>FLGDGGDVSFSTRGTQNWTVERLLQAHRQLEERGYVFVGYHGTFLEAAQSIVFGGVRARSQDLDAIWRGFYIAGDPALAYGYAQDQEPDARGRIRNGALLRVYVPRSSLPGFYRTSLTLAAPEAAGEVERLIG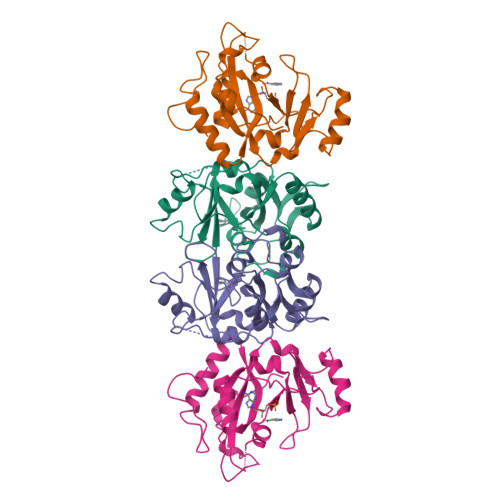HPLPLRLDAITGPEEEGGRLETILGWPLAERTVVIPSAIPTDPRNVGGDLDPSSIPDKEQAISALPDYASQPGKPPREDLK[2x]>[4x]MSISWTRNFFERFCVEEYNIDTIKQSSFLSADLLPSLGARINQSTKLRKHIISPFNPRYRAWEMWLVLLVIYSAWICPFQFAFITYKKDAIFIIDNIVNGFFAIDIILTFFVAYLDSHSYLLVDSPKKIAIRYLSTWFAFDVCSTAPFQPLSLLFNYNGSELGFRILSMLRLWRLRRVSSLFARLEKDIRFNYFWIRCTKLISVTLFAIHCAGCFNYLIADRYPNPRKTWIGAVYPNFKEASLWNRYVTALYWSITTLTTTGYGDFHAENPREMLFDIFFMMFNLGLTAYLIGNMTNLVVHWTSRTRTFRDSVRAASEFASRNQLPHDIQDQMLSHICLKFKTEGLKQQETLNNLPKAIRSSIANYLFFPIVHNIYLFQGVSRNFLFQLVSDIDAEYFPPKEDIILQNEAPTDLYILVSGAVDFTVYVDG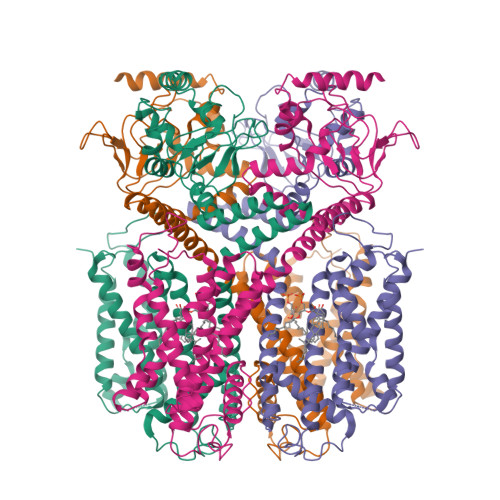HDQFQGKAVIGETFGEVGVLYYRPQPFTVRTTELSQILRISRTSLMSAMHAHADDGRVIMNNLFMKLRGQQSSRGSLEVLFQ> SCESSMVLGYWDIRGLAHAIRLLLEFTDTSYEEKRYTCGEAPDYDRSQWLDVKFKLDLDFPNLPYLLDGKNKITQSNAILRYIARKHNMCGETEEEKIRVDIIENQVMDFRTQLIRLCYSSDHEKLKPQYLEEL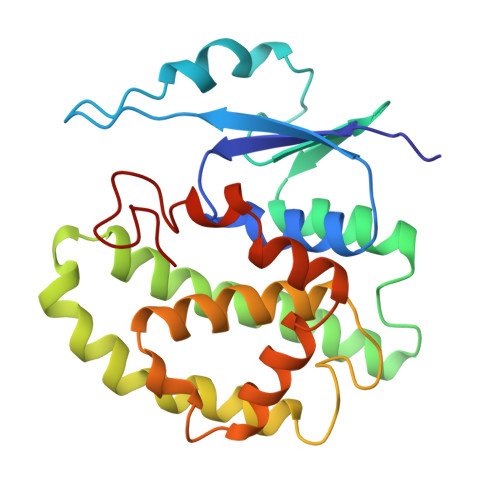PGQLKQFSMFLGKFSWFAGEKLTFVDFLTYDILDQNRIFDPKCLDEFPNLKAFMCRFEALEKIAAYLQSDQFCKMPINNKMAQWGNKPVC>[2x]TKDLPIHACSYCGIHDPACVVYCNTSKKWFCNGRGNTSGSHIVNHLVRAKCKEVTLHKDGPLGETVLECYNCGCRNVFLLGFIPAKADSVVVLLCRQPCASQSSLKDINWDSSQWQPLIQDRCFLSWLVKIPSEQEQLRARQITAQQINKLEELWKENPSATLEDLEKPGVDEEPQHVLLRYEDAYQYQNIFGPLVKLEADYDKKLKESQTQDNITVRWDLGLNKKRIAYFTLPKTDSDMRLMQGDEICLRYKGDLAPLWKGIGHVIKVPDNYGDEIAIELRSSVGAPVEVTHNFQ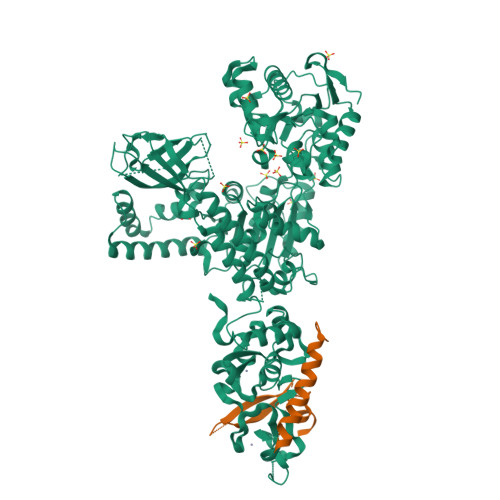VDFVWKSTSFDRMQSALKTFAVDETSVSGYIYHKLLGHEVEDVIIKCQLPKRFTAQGLPDLNHSQVYAVKTVLQRPLSLIQGPPGTGKTVTSATIVYHLARQGNGPVLVCAPSNIAVDQLTEKIHQTGLKVVRLCAKSREAIDSPVSFLALHNQIRNMDSMPELQKLQQLKDETGELSSADEKRYRALKRTAERELLMNADVICCTCVGAGDPRLAKMQFRSILIDESTQATEPECMVPVVLGAKQLILVGDHCQLGPVVMCKKAAKAGLSQSLFERLVVLGIRPIRLQVQYRMHPALSAFPSNIFYEGSLQNGVTAADRVKKGFDFQWPQPDKPMFFYVTQGQEEIASSGTSYLNRTEAANVEKITTKLLKAGAKPDQIGIITPYEGQRSYLVQYMQFSGSLHTKLYQEVEIASVDAFQGREKDFIILSCVRANEHQGIGFLNDPRRLNVALTRARYGVIIVGNPKALSKQPLWNHLLNYYKEQKVLVEGPLNNLRESLMQFS;>[2x]AMGVPCVEDEDFIQALDKMMLENLQQRSGESVKVHQLDVAIPLHLKSQLRKGPPLGGGEGEAESADTMPFVMLTRKGNKQQFKILNVPMSSQLAANH>[2x]GAMAAGVKQLADDRTLLMAGVSHDLRTALTRIRLATEMMSEQDGYLAESINK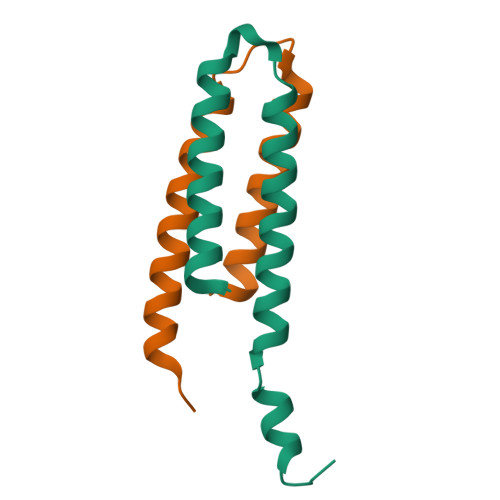DIEECNAIIEQFIDYLR(1R,4S,6R)-6-({[2-(ACETYLAMINO)-2-DEOXY-ALPHA-D-GLUCOPYRANOSYL]OXY}METHYL)-4-HYDROXY-1-{[(15-METHYLHEXADECANOYL)OXY]METHYL}-4-OXIDO-7-OXO-3,5-DIOXA-8-AZA-4-PHOSPHAHEPTACOS-1-YL 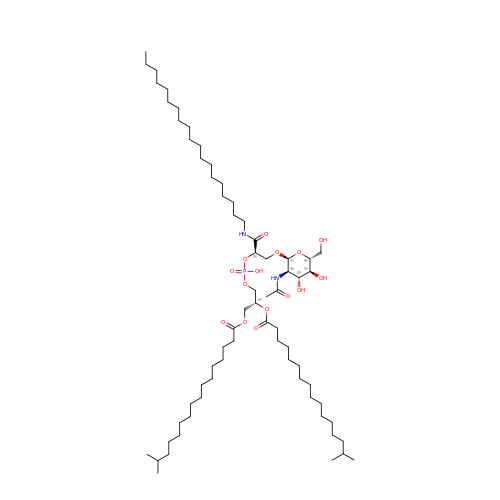15-METHYLHEXADECANOATE | C67 H129 N2 O15 P | LEQHPGOQHCQGAI-TYASGWLASA-N> MGSSHHHHHHSSGLVPRGSDLQE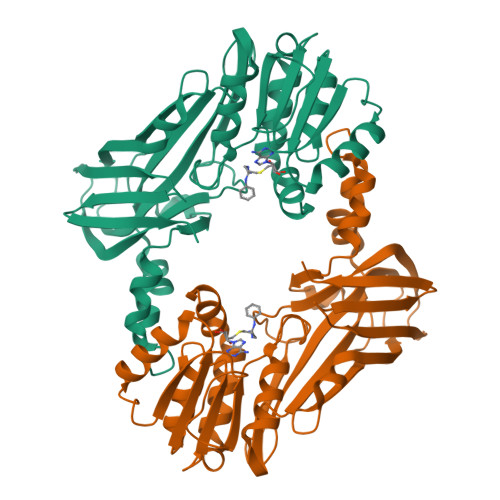DEDGVYFSSYGHYGIHEEMLKDKIRTESYRDFIYQNPHIFKDKVVLDVGCGTGILSMFAAKAGAKKVLGVDQSEILYQAMDIIRLNKLEDTITLIKGKIEEVHLPVEKVDVIISEWMGYFLLFESMLDSVLYAKNKYLAKGGSVYPDICTISLVAVSDVNKHADRIAFWDDVYGFKMSCMKKAVIPEAVVEVLDPKTLISEPCGIKHIDCHTTSISDLEFSSDFTLKITRTSMCTAIAGYFDIYFEKNCHNRVVFSTGPQSTKTHWKQTVFLLEKPFSVKAGEALKGKVTVHKNKKDPRSLTVTLTLNNSTQTYGLQ>[2x]MSGTGRLAGKIALITGGAGNIGSELTRRFLAEGATVIISGRNRAKLTALAERMQAEAGVPAKRIDLEVMDGSDPVAVRAGIEAIVARHGQIDILVNNAGSAGAQRRLAEIPLTEAELGPGAEETLHASIANLLGMGWHLMRIAAPHMPVGSAVINVSTIFSRAEYYGRIPYVTPKAALNALSQLAARELGARGIRVNTIFPGPIESDRIRTVFQRMDQLKGRPEGDTAHHFLNTMRLCRANDQGALERRFPSVGDVADAAVFLASAESAALSGET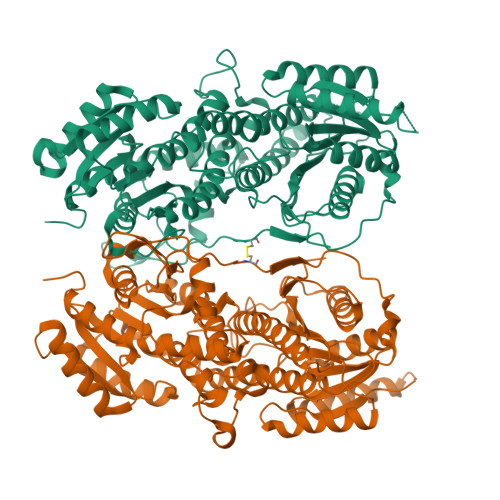IEVTHGMELPACSETSLLARTDLRTIDASGRTTLICAGDQIEEVMALTGMLRTCGSEVIIGFRSAAALAQFEQAVNESRRLAGADFTPPIALPLDPRDPATIDAVFDWAGENTGGIHAAVILPATSHEPAPCVIEVDDERVLNFLADEITGTIVIASRLARYWQSQRLTPGARARGPRVIFLSNGADQNGNVYGRIQSAAIGQLIRVWRHEAELDYQRASAAGDHVLPPVWANQIVRFANRSLEGLEFACAWTAQLLHSQRHINEITLNIPANI> GPDSMPGDHRRIRGPEESQPPQLYAADEEEAPGTRDPTRLRPVYARAGLLSQAKGSAYLEAGGTKVLCAVSGPRQAEGGERGGGPAGAGGEAPAALRGRLLCDFRR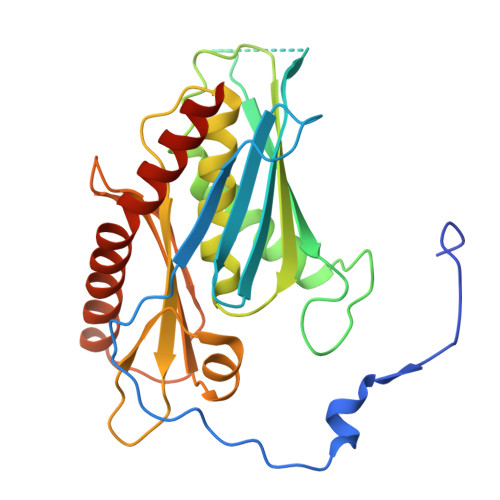APFAGRRRRAPPGGCEERELALALQEALEPAVRLGRYPRAQLEVSALLLEDGGSALAAALTAAALALADAGVEMYDLVVGCGLSLAPGPAPTWLLDPTRLEEERAAAGLTVALMPVLNQVAGLLGSGEGGLTESWAEAVRLGLEGCQRLYPVLQQSLVRAARRRGAAAQP N-({4-methyl-2-[4-(trifluoromethyl)phenyl]-1,3-thiazol-5-yl}carbonyl)-L-serine 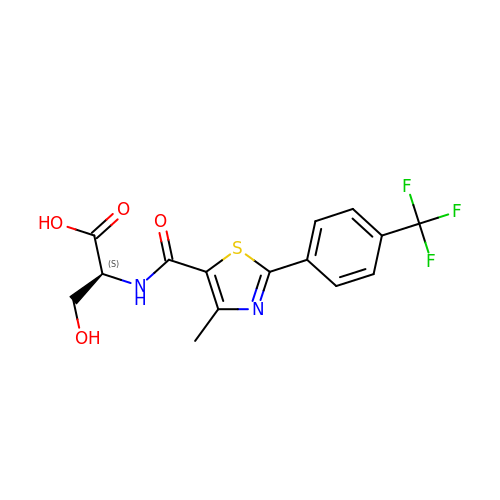| C15 H13 F3 N2 O4 S | YJGBVICLINVYSP-UHFFFAOYSA-N>MAALIAENF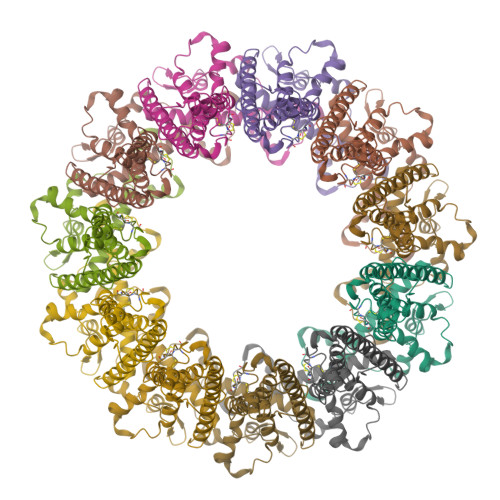RFLSLFFKSKDVMIFNGLVALGTVGSQELFSVVAFHCPCSPARNYLYGLAAIGVPALVLFIIGIILNNHTWNLVAECQHRRTKNCSAAPTFLLLSSILGRAAVAPVTWSVISLLRGEAYVCALSEFVDPSSLTAREEHFPSAHATEILARFPCKENPDNLSDFREEVSRRLRYESQLFGWLLIGVVAILVFLTKCLKHYCSPLSYRQEAYWAQYRANEDQLFQRTAEVHSRVLAANNVRRFFGFVALNKDDEELIANFPVEGTQPRPQWNAITGVYLYRENQGLPLYSRLHKWAQGLAGNGAAPDNVEMALLPSENLYFQ[11x]>[4x]MSLLAKIVDGKNLSFEEAYELFNELKGSDGVLIGAYLAALQTKGYTGEELAGLARAMRDSAVKLDLGKVADTAGTGGDGSSTINVSTASALILSAFTRVAKHGNVSITSKSGSANVLEALGLNIRVSPERAREMVESTNFTFIFAPAYHPALRPIMPVRKALGIKTVFNVIGPLANPADPAYQVVGVNSPELLEPVAEALEFLGVERALVVHGSGMDEVSPHRETLVLEVGNGVERYTLSPEDF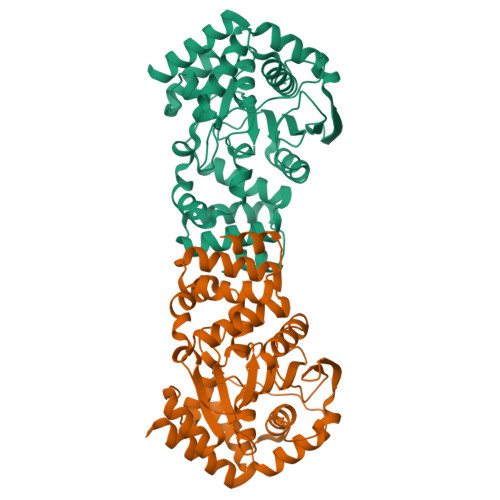GIEPVKPLPCSSPEESAARIKAVLGGSGRREDRDFILVNASAALYASGVAEDFREGLEMAREALGQGMLEKLEEIACLSKS> MELPTYRYPLELDTANNRVQVADRFGMRTGTWTGQLQYQHPQLSWRANVTLNLM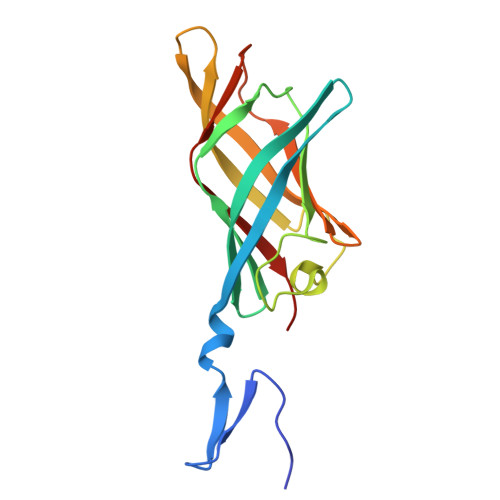KVDDWLVLSFSQMTTNSIMADGKFVINFVSGLSSGWQTGDTEPSSTIDPLSTTFAAVQFLNNGQRIDAFRIMGVSEWTDGELEIKNYGGTYTGHTQVYWAPWTIMYPCNVR> MASSGVAGGRQAEDTLQPPPELLPESKPPPPPQPLPVAALPPPAAPRPQSPAGAKEENYSFLPLVHNVIKCMDKDSPDLHQDLNALKTKFQELRKLIGTMPGIHVSPEQQQQQLHSLREQVRTKNELLQKYKSL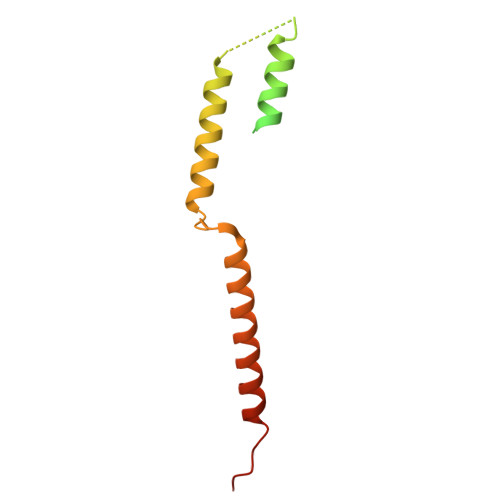CMFEIPKD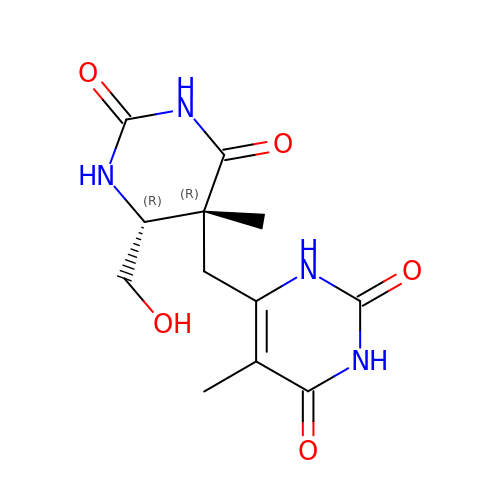6-{[4-(HYDROXYMETHYL)-5-METHYL-2,6-DIOXOHEXAHYDROPYRIMIDIN-5-YL]METHYL}-5-METHYLPYRIMIDINE-2,4(1H,3H)-DIONE | C12 H16 N4 O5 | KBBKHMIEEMSXSM-JVXZTZIISA-N> NLQNIIYNPVIPFVGTIPDQLDPGTLIVIRGHVPSDADRFQVDLQNGSSM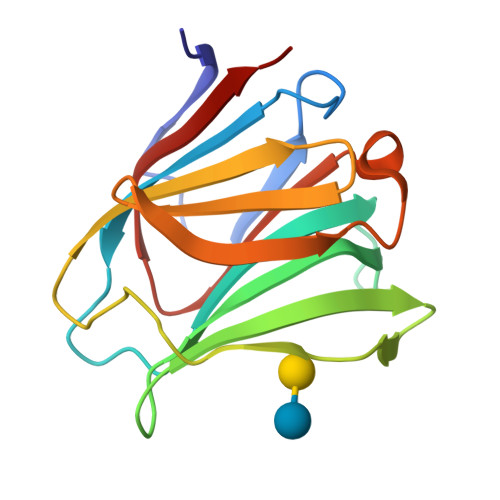KPRADVAFHFNPRFKRAGCIVCNTLINEKWGREEITYDTPFKREKSFEIVIMVLKDKFQVAVNGKHTLLYGHRIGPEKIDTLGIYGKVNIHSIGFSFS> IVGGYTCGANTVPYQVSLNSG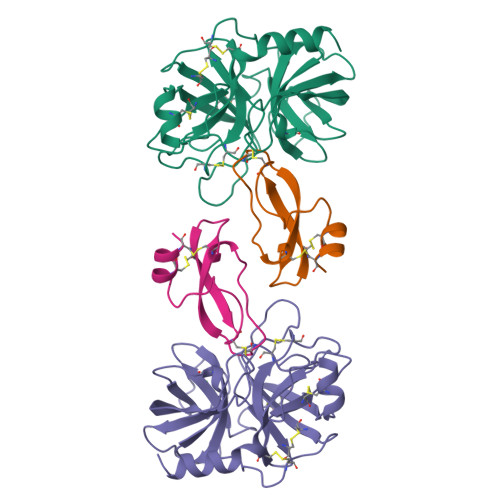YHFCGGSLINSQWVVSAAHCYKSGIQVRLGEDNINVVEGNEQFISASKSIVHPSYNSNTLNNDIMLIKLKSAASLNSRVASISLPTSCASAGTQCLISGWGNTKSSGTSYPDVLKCLKAPILSTSSCKSAYPGQITSNMFCAGYLEGGKDSCQGDSGGPVVCSGKLQGIVSWGSGCAQKNKPGVYTKVCNYVSWIKQTIASN;> VREVCSEQAETGPCRAMISRWYFDVTEGKCAPFFYGGCGGNRNNFDTEEYCMAVCGSA>MLDEKSSNTASVVVLCTAPDEATAQDLAAKVLAEKLAACATLIPGATSLYYWEGKLEQEYEVQMILKT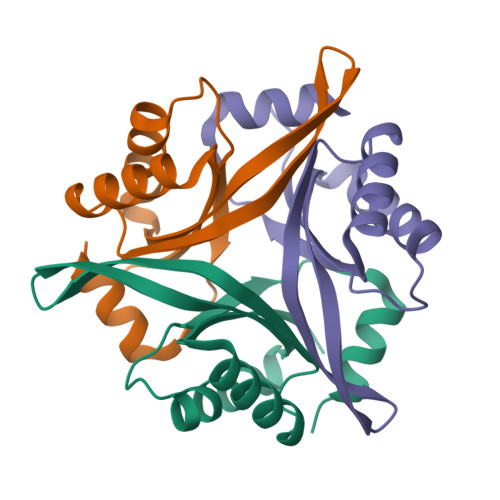TVSHQQALLECLKSHHPYQTPELLVLPVTHGDTDYLSWLNASLR[6x]N-[(1S)-2-(hydroxyamino)-1-(3-methoxy-1,1-dioxo-1lambda~6~-thietan-3-yl)-2-oxoethyl]-4-(6-hydroxyhexa-1,3-diyn-1-yl)benzamide | C19 H20 N2 O7 S | 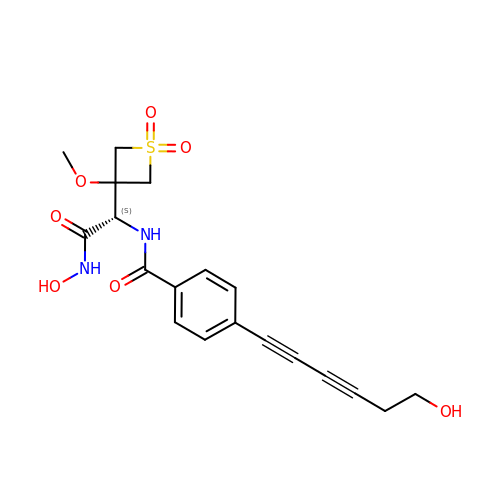QVQHZORAUGAARX-MRXNPFEDSA-N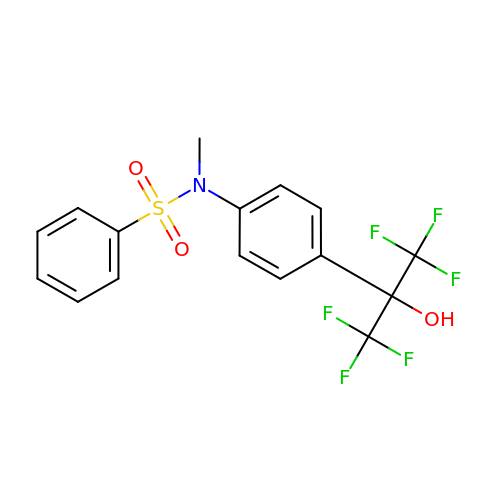N-[4-(1,1,1,3,3,3-hexafluoro-2-hydroxypropan-2-yl)phenyl]-N-methylbenzenesulfonamide | C16 H13 F6 N O3 S | CNVKZYLQZYULJV-UHFFFAOYSA-N> LVHVASVEKGRSYEDFQKVYNAIALKLREDDEYDNYIGYGPVLVRLAWHISGTWDKHDNTGGS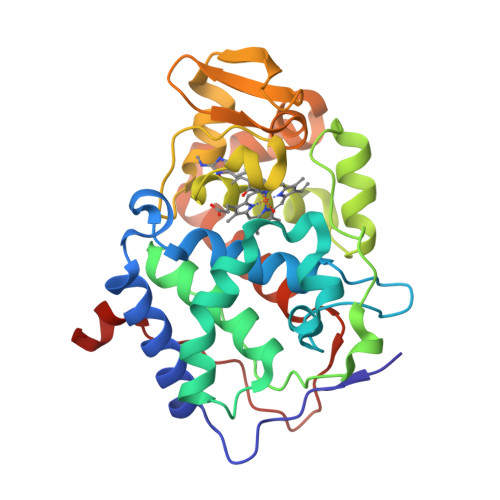YGGTYRFKKEFNDPSNAGLQNGFKFLEPIHKEFPWISSGDLFSLGGVTAVQEMQGPKIPWRCGRVDTPEDTTPDNGRLPDADKDAGYVRTFFQRLNMNDREVVALMGAHALGKTHLKNSGYEGGGANNVFTNEFYLNLLNEDWKLEKNDANNEQWDSKSGYMMLPTDYSLIQDPKYLSIVKEYANDQDKFFKDFSKAFEKLLENGITFPKDAPSPFIFKTLEEQGL> MASVHGTTYELLRRQGIDTVFGNPGSNELPFLKDFPEDFRYILALQEACVVGIADGYAQASRKPAFINLHSAAGTGNAMGALSNAWNSHSPLIVTAGQQTRAMIGVEALLTNVDAANLPRPLVKWSYEPASAAEVPHAMSRAIHMASMAPQGPVYLSVPYDDWDKDADPQSHHLFDRHVSSSVRLNDQDLDILVKALNSASNPAIVLGPDVDAANANADCVMLAERLKAPVWVAPSAPRCPFPTRHPCFRGLMPAGIAAISQLLEGHDVVLVIGAPVFRYHQYDPGQYLKPGTRLISVTCDPLEAARAPMGDAIVADIGAMASALANLVEESSRQLPTAAPEPAKVDQDAGRLHPETVFDTLNDMAPENAIYLNESTSTTAQMWQRLNMRNPGSYYFCAAGGLGFALPAAIGVQLAEPERQVIAVIGDGSANYSISALWTAAQYNIPTIFVIMNNGTYGALRWFAGVLEAENVPGLDVPGIDFRALAKGYGVQALKADNLEQLKGSLQE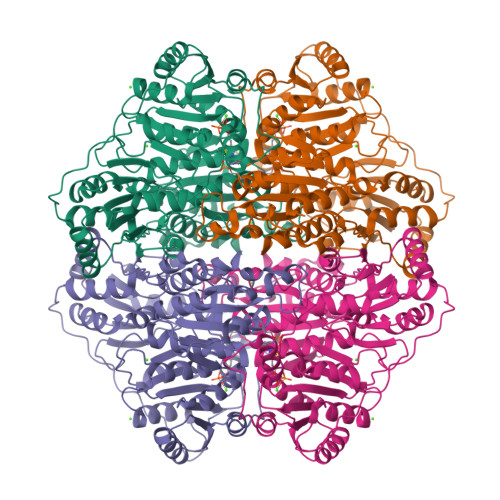ALSAKGPVLIEVSTVSPVK> KPKNKDKDKKVPEPDNKKKKPKKEEEQKWKWWEEERYPEGIKWKFLEHKGPVFAPPYEPLPENVKFYYDGKVMKLSPKAEEVATFFAKMLDHEYTTKEIFRKNFFKDWRKEMTNEEKNIITNLSKCDFTQMSQYFKAQTEARKQMSKEEKLKIKEENEKLLKEYGFCIMDNH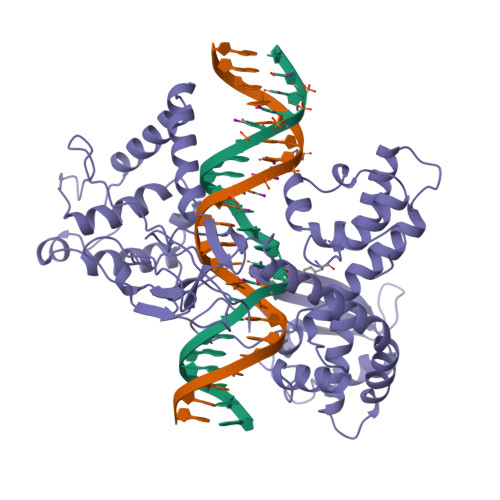KERIANFKIEPPGLFRGRGNHPKMGMLKRRIMPEDIIINCSKDAKVPSPPPGHKWKEVRHDNKVTWLVSWTENIQGSIKYIMLNPSSRIKGEKDWQKYETARRLKKCVDKIRNQYREDWKSKEMKVRQRAVALYFIDKLALRAGNEKEEGETADTVGCCSLRVEHINLHPELDGQEYVVEFDFLGKDSIRYYNKVPVEKRVFKNLQLFMENKQPEDDLFDRLNTGILNKHLQDLMEGLTAKVFRTYNASITLQQQLKELTAPDENIPAKILSYNRANRAVAILCNHQRAPPKTFEKSMMNLQTKIDAKKEQLADARRDLKSAKADAKVMKDAKTKKVVESKKKAVQRLEEQLMKLEVQATDREENKQIALGTSKLNYLDPRITVAWCKKWGVPIEKIYNKTQREKFAWAIDMADEDYEF> GPLGSQLIQEFTAAQRRGEIGRMREVAAVLLHFKGYAHCVDVYIKQCQEGAYMRNDVFEDIAILCQRVNKQVGEVFCSPETVMAKLIQSIFENKIQAHVKERLDETRNSDVEQYLKNLYDLYTRTTALAAKLTDYNLGSDKHTFLSKLIKNIFSCYLESYIDMERQYLQNRSGMILQRYYDSKNH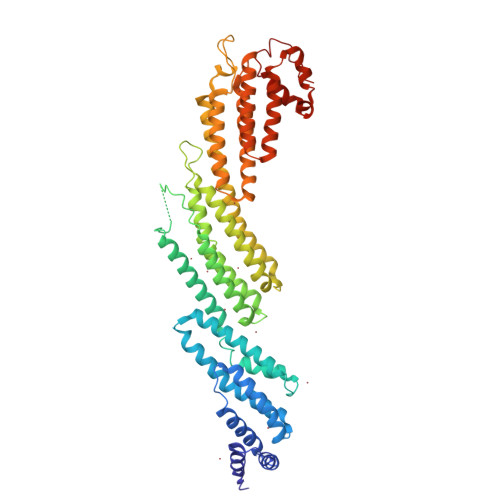QKRPVGTGSITNLPLGPSIDTHGETLLSQEVVVNLLQETRHAFERCNKLSDPADLPKNAFSIFLILVEYLCVDHIDYALEIGLSAIPSADAKNANLYFLDVVQQANTIFHLFDKQFNDHLMPLISSSPKLTECLHKKKEVIEQMEVKLDTGIDRTLNCMIGQMKYILTTEQKKTDFKPEDENNVMIQYTTACSKVCAYVGKQVERVRRSMDGKNVDTVLTELGVRFHRLIHEHLQQFSYSSMGGMLAICDVAEYRRSAKDFRVPLVLQLFDTLHALCNLLVVAPDNLKQVCSGEQLTNLDRNLLHAFVQLRVDYRSARLGRHFS>[2x]QFTL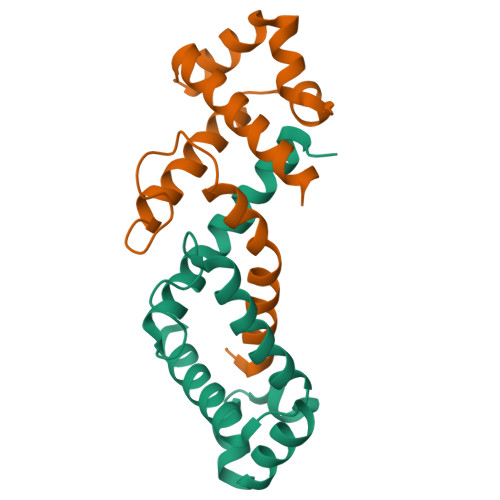RDMYEQFQNIMKMGPFSQILGMIPGFGTDFMSKGNEQESMARLKKLMTIMDSMNDQELDSTDGAKVFSKQPGRIQRVARGSGVSTRDVQELLTQYTKFAQMVKKM>MGGHHHHHHGENLYFQGISSETGEMGILWEFDPIINKWIRLSMKLKVERKPFAEGALREAYHTVSLGVGTDENYPLGTTTKLFPPIEMISPISKNNEAMTQLKNGTKFVLKLYKKEAEQQASRELYFEAVKMQMVCRDWGNKFNQKKPPKKIEFLMSWVVELIDRSPSSNGQPILCSIEPLLVGEFKKNNSNYGAVLTNRSTPQAFSHFTYELSNKQMIVVDIQGVDDLYTDPQIHTPDGKGFGLGNLGKAGINKFITTHKCNAVCALLDLDVKLGGVLS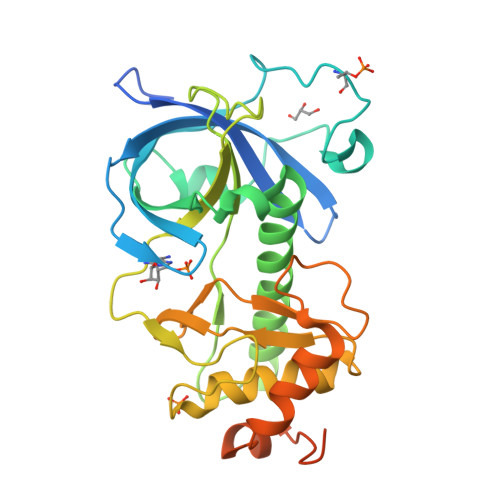GNNNQQLQQGTMVKADILPELMPSDNT[2x]>MAETAPLRVQLIAKTDFLAPPDVPWTTDADGGPALVEFAGRACYQSWSKPNPKTATNAGYLRHIIDVGHFSVLEHASVSFYITGISRSCTHELIRHRHFSYSQLSQRYVPEKDSRVVVPPGMEDDADLRHILTEAADAARATYSELLA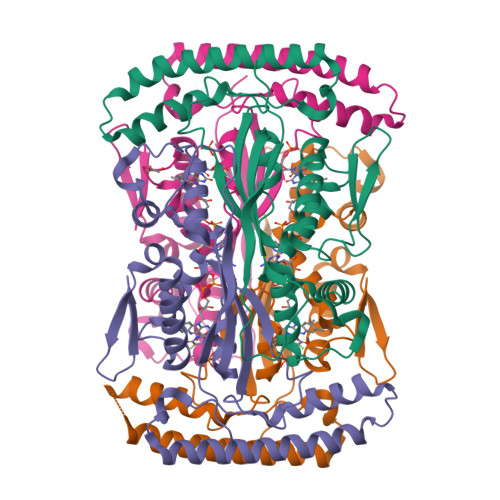KLEAKFADQPNAILRRKQARQAARAVLPNATETRIVVTGNYRAWRHFIAMRASEHADVEIRRLAIECLRQLAAVAPAVFADFEVTTLADGTEVATSPLATEALEHHHHHH[8x]>SNANEAQQYYLDADEAEAWIGEQELYVISDEIPKDEEGAIVMLKRHLRQQRAVEDYGRNIKQLASRAQGLLSAGHPEGEQIIRLQGQVDKHYAGLKDVACERKRKLENMYHLFQLKRETDDLEQWISEKELVASSPEMGQDFDHVTLLRDKFRDFARETGAIGQERVDNVNAFIERLIDAGHSEAATIAEWKDGLNEMWADLLELIDTRMQLLAASYDLHRYFYTGAEILGLIDEKHRELPEDVGLDASTAESFHRVHTAFERDVHLLGVQVQQFQDVATRLQTAYAGEKAEAIQNKEQEVSAAWQALLDACAGRRTQLVDTADKF[2x];>[2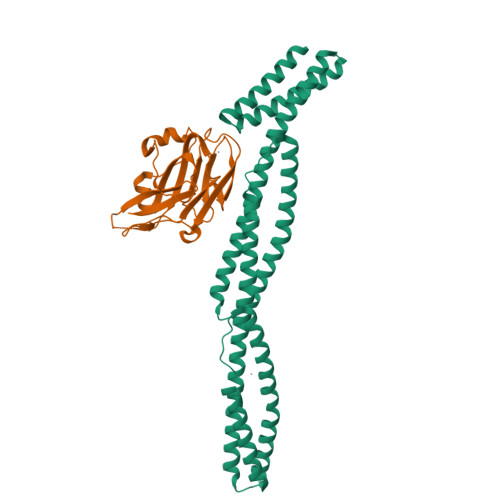x]SNATGFLVSFMVDARGGSMRGSRHNGLRVVIPPRTCAAPTRITCRLVKPQKLSTPPPLAEEEGLASRIIALGPTGAQFLSPVIVEIPHFASHGRGDRELVVLRSENGSVWKEHRSRYGESYLDQILNGMDEELGSLEELEKKRVCRIITTDFPLYFVIMSR~{N}-(pyridin-2-ylmethyl)-2-(2-thiophen-2-ylindol-1-yl)ethanamide | C20 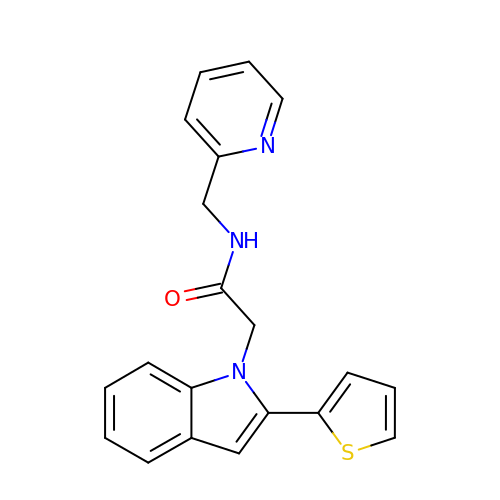H17 N3 O S | HTRIQCMSXMSDKF-UHFFFAOYSA-N> THPVEAAERNYERARAELNQANEDVARNQERQAKAVQVYNSRKSELDAANKTLADAIAEIKQFNRFAHDPMAGGHRMWQMAGLKAQRA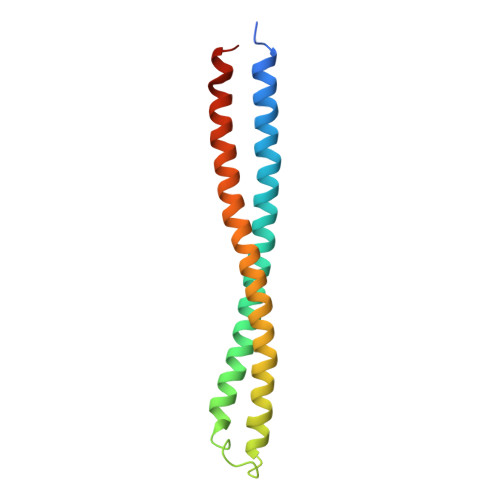QTDVNNKQAAFDAAAKEKSDADAALSAAQERRKQKENKEKDAKDKLD>[4x]MENKIIYFLCTGNSCRSQMAEGWA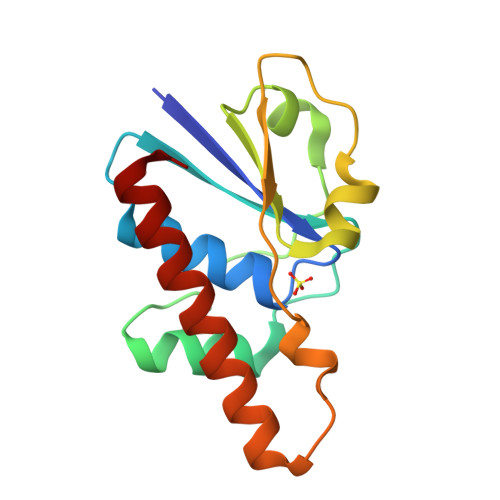KQYLGDEWKVYSAGIEAHGLNPNAVKAMKEVGIDISNQTSDIIDSDILNNADLVVTLCGDAADKCPMTPPHVKREHWGFDDPARAQGTEEEKWAFFQRVRDEIGNRLKEFAETGK> MENTENSVDSKSIKNLEPKIIHGSESMDSGISLDNSYKMDYPEMGLCIIINNKNFHKSTGATSRSGTDVDAANLRETFRNLKYEVRNKNDLTREEIVELMRDVSKEDHSKRSSFVCVLLSHGEEGIIFGTNGPVDLK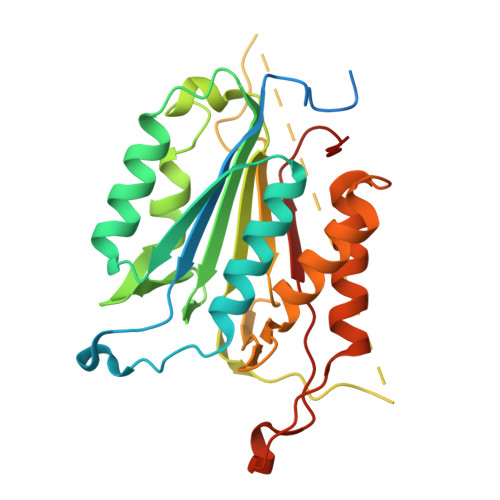KITNFFRGDRCRSLTGKPKLFIIQACRGTELDCGIETDSGVDDDMACHKIPVEADFLYAYSTAPGYYSWRNSKDGSWFIQSLCAMLKQYADKLEFMHILTRVNRKVATEFESFSFDATFHAKKQIPCIVSMLTKELYFYH Human cellular retinol binding protein II (hCRBPII) was used as a protein engineering platform to rationally regulate absorptive and emissive properties of a covalently bound fluorogenic dye. We demonstrate the binding of a thio-dapoxyl analog via formation of a protonated imine between an active site lysine residue and the chromophore’s aldehyde. Previously, we showed the utility of human cellular retinol-binding protein II (hCRBPII) mutants as a fluorophoric tag, wherein an active site lysine residue (Q108K) reacts with synthetic aldehydic chromophores, giving rise to the formation of either an imine (Schiff base, SB) or an iminium (protonated SB, PSB). Q108K functions as the active-site lysine and forms a Schiff base with the aldehyde, whereas the K40L mutation is assumed to eliminate interactions between Q108K and Lys40, an interaction that could otherwise impede imine formation, and is also required to promote Schiff base protonation.

Gratifyingly, the red shifting properties of T51V and T53S to M1 were additive, resulting in 47 and 23 nm, absorption and emission red shifts, respectively (M8). Thus, the M8 template (Q108 K:K40L:T51V:T53S) was retained for further protein engineering. We first focused on the Arg58 position, introducing aromatic residues (M9-M12) to the parent tetramutant M8. However, results were disappointing with most mutations resulting in modest hypsochromic wavelength shifts. Nonetheless, we were able to successfully obtain a crystal structure of M11, which guided further engineering efforts. The tryptophan at position 58 does not sequester the binding pocket; instead, it flips inside, where it makes a cation - π interaction with the diethyl-amino group of TD-1V (3.7 Å). Additionally, comparison of the M10 and M11 structures shows that introduction of Trp58 results in an almost 90° rotation of the entire chromophore, altering the position and therefore interactions of the imine at the opposite end. A conserved water network connecting the hydroxyl group of Tyr19 and the thiophene sulfur atom of TD-1V was observed in the M11 crystal structure. The explanation for why only the combination of Y19W with R58W led to the significant change in spectral shift as opposed to the combination of R58H and Y19W is probably due to the nearly 90° rotation of the chromophore trajectory enforced by its interaction with Trp58 for M11.

>[2x]TRDQNGTWEMESNENFEGYMKALDIDFATRKIAVRLTQTLVIDQDGDNFKVKSTSTFWNYDVDFTVGVEFDEYTKSLDNRHVKALVTWEGDVLVCVQKGEKENRGWKKWIEGDKLYLELTCGDQVCRQVFKKK>[2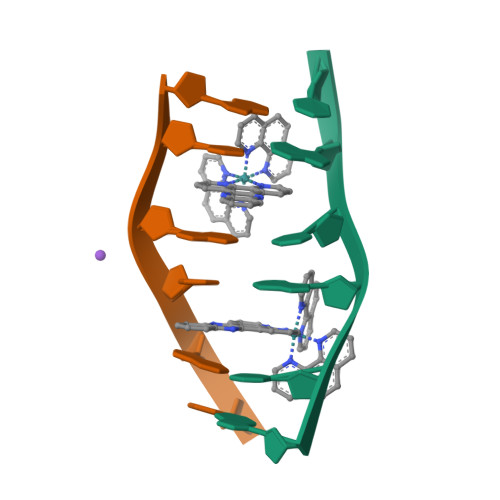x]ATGCAT> MSKQRVFIAGHRGMVGSAIRRQLEQRGDVELVLRTRDELNL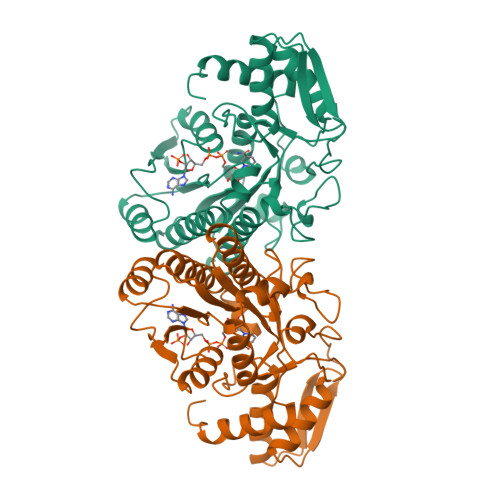LDSRAVHDFFASERIDQVYLAAAKVGGIVANNTYPADFIYQNMMIESNIIHAAHQNDVNKLLFLGSSCIYPKLAKQPMAESELLQGTLEPTNEPYAIAKIAGIKLCESYNRQYGRDYRSVMPTNLYGPHDNFHPSNSHVIPALLRRFHEATAQNAPDVVVWGSGTPMREFLHVDDMAAASIHVMELAHEVWLENTQPMLSHINVGTGVDCTIRELAQTIAKVVGYKGRVVFDASKPDGTPRKLLDVTRLHQLGWYHEISLEAGLASTYQWFLENQDRFRG> MTILTDENYVDIAEKAILKLERNTRNRKNPDAFFLTTSKLRNLLSLTSTLFDESKVKEYDALLDRIAYLRVQFVYQAGREIAVKDLIEKAQILEALKEIKDRE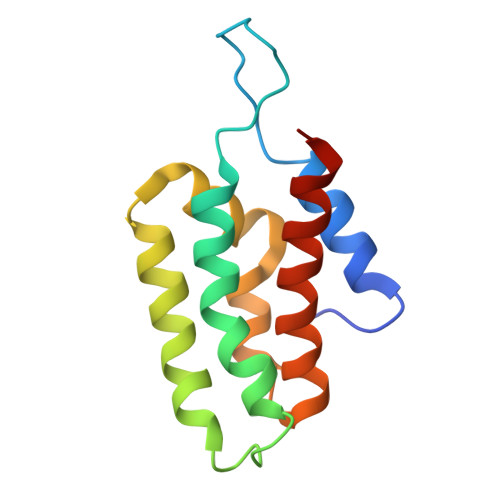TLQRFCRYMEALVAYFKFYGGKD>[2x]SNAMIAKEFETFLLGQEETFLTPAKNLAVLIDTHNADHATLLLSQMTYT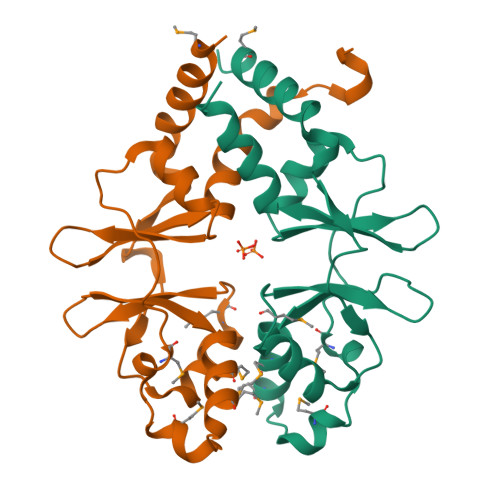RVPVVTDEKQFVGTIGLRDIMAYQMEHDLSQEIMADTDIVHMTKTDVAVVSPDFTITEVLHKLVDESFLPVVDAEGIFQGIITRKSILKAVNALLHDFSKEYEIRCQ>EGDIHMKKGYHHHHHLVPRGSAPYASLTEIEHLVQSVCKSYRETCQLRLEDLLRQRSNIFSREEVTGYQRKSMWEMWERCAHHLTEAIQYVVEFAKRLSGFMELCQNDQIVLLKAGAMEVVLVRMCRAYNADNRTVFFEGKYGGMELFRALGCSELISSIFDFSHSLSALHFSEDEIALYTALVLINAHRPGLQEKRKVEQLQYNLELAFHHHLEKT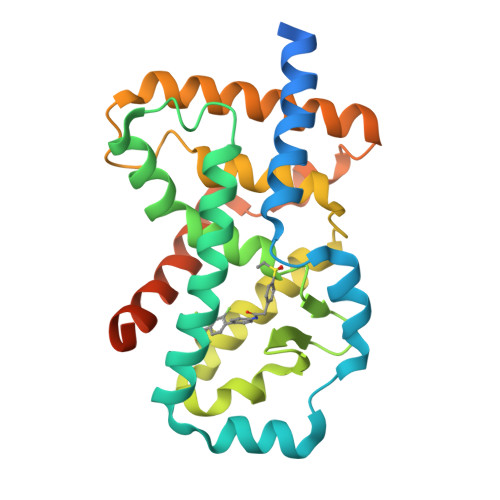HRQSILAKLPPKGKLRSLCSQHVERLQIFQHLHPIVVQAAFPPLYKELFS[3x]>[2x]MLELVEEHRCFSGVQRTYKHDSQTIGLPMRFSVFLPPQAAHGKVPALFYLAGLTCTEETFAIKAGAQRFASEHGIALIGPDTSPRGAGVPNEGAAWDFGVGAGFYVDATQEPWARNYRMYSYVTQELRTTVLAELPVREDRLGIFGHSMGGHGALVLALRNPDIYKSVSAFAPI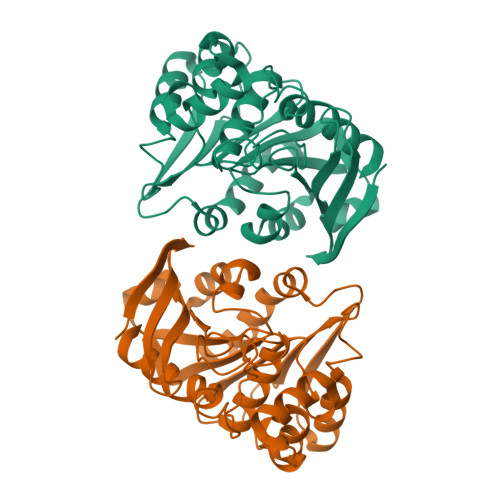AAPSHCPWGEKAFSGYLGDDRETWKQYDASELVKSAKTKFDAGILIDQGLADNFLATQLHPEIFEAAAKAAGQAVTLRRHEGYDHGYYFISTFIGEHVAFHARTLCA> GPAMHEFVSGTPG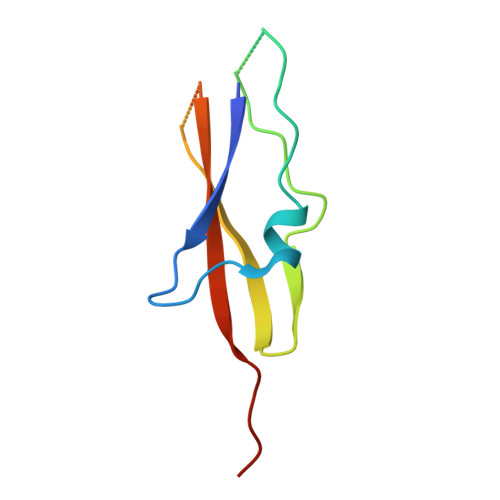KELPQEVKDLLPADQTDLKDGSQSTPTQPSKTEVKTAEGTWSFKSYDKTSETINEADVHFVGTWEFTPAPTYKAT>MSREEVESLIQEVLEVYPEKARKDRNKHLAVNDPAVTQSKKCIISNKKSQPGLMTIRGCAYAGSKGVVWGPIKDMIHISHGPVGCGQYSRAGRRNYYIGTTGVNAFVTMNFTSDFQEKDIVFGGDKKLAKLIDEVETLFPLNKGISVQSECPIGLIGDDIESVSKVKGAELSKTIVPVRCEGFRGVSQSLGHHIANDAVRDWVLGKRDEDTTFASTPYDVAIIGDYNIGGDAWSSRILLEEMGLRCVAQWSGDGSISEIELTPKVKLNLVHCYRSMNYISRHMEEKYGIPWMEYNFFGPTKTIESLRAIAAKFDESIQKKCEEVIAKYKPEWEAVVAKYRPRLEGKRVMLYIGGLRPRHVIGAYEDLGMEVVGTGYEFAHNDDYDRTMKEMGDSTLLYDDVTGYEFEEFVKRIKPDLIGSGIKEKFIFQKMGIPFREMHSWDYSGPYHGFDGFAIFARDMDMTLNNPCWKKLQAPWE[2x];>SQQVDKIKASYPLFLDQDYKDMLAKKRDGFEEKYPQDKIDEVFQWTTTKEYQELNFQREALTVNPAKACQPLGAVLCALGFEKTMPYVHGSQGCVAYFRSYFNRHFREPVSCVSDSMTEDAAVFGGQQNMKDGLQNCKATYKPDMIAVSTTCMAEVIGDDLNAFINNSKKEGFIPDEFPVPFAHTPSFVGSHVTGWDNMFEGIARYFTLKSMDDKVVGSNKKINIVPGFETYLGNFRVIKRMLSEMGVGYSLLSDPEEVLDTPADGQFRMYAGGTTQEEMKDAPNALNTVLLQPWHLEKTKKFVEGTWKHEVPKLNIPMGLDWTD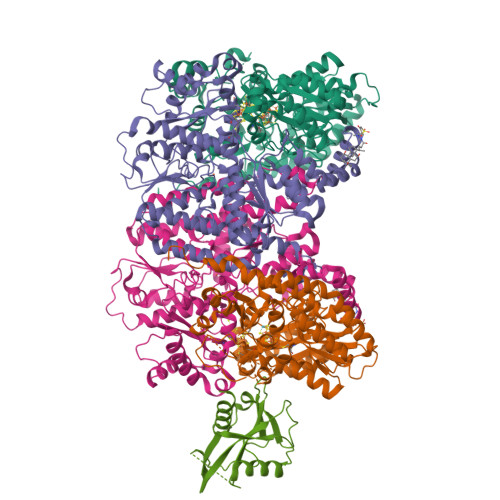EFLMKVSEISGQPIPASLTKERGRLVDMMTDSHTWLHGKRFALWGDPDFVMGLVKFLLELGCEPVHILCHNGNKRWKKAVDAILAASPYGKNATVYIGKDLWHLRSLVFTDKPDFMIGNSYGKFIQRDTLHKGKEFEVPLIRIGFPIFDRHHLHRSTTLGYEGAMQILTTLVNSILERLDEETRGMQATDYNHDLVR[2x];> MSWRILLCHKHPVSARLRFLIPTGGGVVLPQTLPRLAVIAEDQEAPVQCHPASALRALQETMALGWQLELIGEFRLNMEVPGQIMPIYLAALAGHELPPPPEGTRWIELTQSIGMPWLDRELLRRVYEELIG> LQ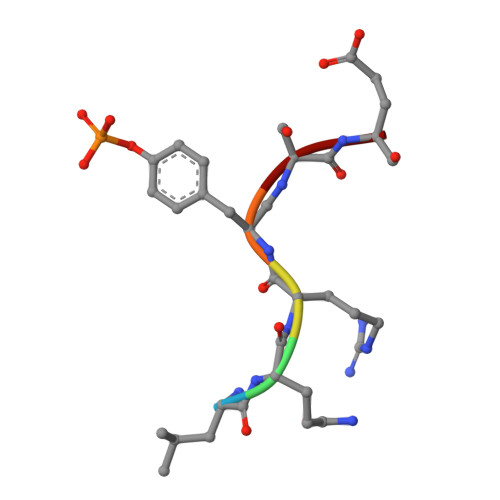RYSE> MERNKLARQII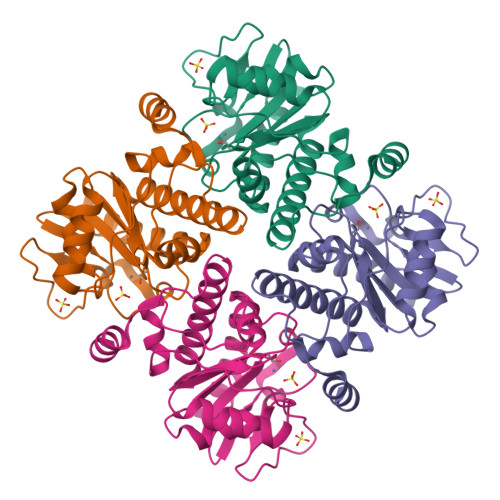DTCLEMTRLGLNQGTAGNVSVRYQDGMLITPTGIPYEKLTESHIVFIDGNGKHEEGKLPSSEWRFHMAAYQSRPDANAVVHNHAVHCTAVSILNRSIPAIHYMIAAAGGNSIPCAPYATFGTRELSEHVALALKNRKATLLQHHGLIACEVNLEKALWLAHEVEVLAQLYLTTLAITDPVPVLSDEEIAVVLEKFKTYGLRIAE>[2x]MSFSCPLCHQPLSREKNSYICPQRHQFDMAKEGYVNLLPVQHKRSRDPGDSAEMMQARRAFLDAGHYQPLRDAIVAQLRERLDDKATAVLDIGCGEGYYTHAFADALPEITTFGLDVSKVAIKAAAKRYPQVTFCVASSHRLPFSDTSMDAIIRIYAPCKAEELARVVKPGGWV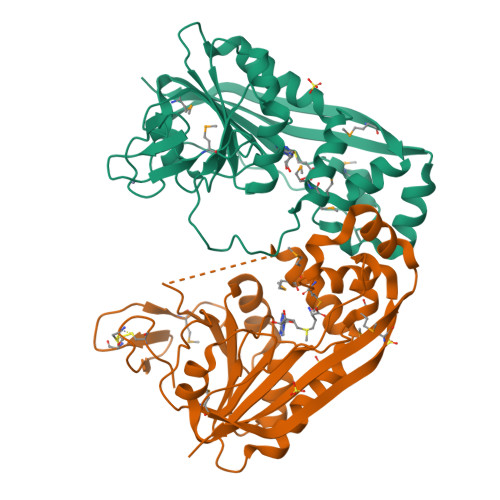ITATPGPRHLMELKGLIYNEVHLHAPHAEQLEGFTLQQSAELCYPMRLRGDEAVALLQMTPFAWRAKPEVWQTLAAKEVFDCQTDFNIHLWQRSY>[2x]MAGRTRIPFNGVGTSVLPAYQTLSAGQYLLSPNQRFKLLLQGDGNLVIQDNGATVWVANEQQPFSSTIPLRNKKAPLAFYVQ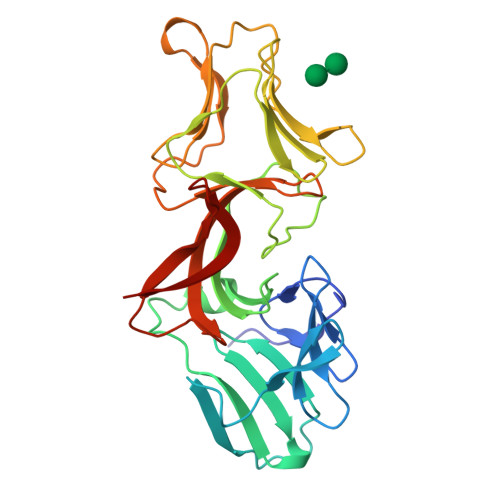YGAFLDDYSRRRVWLTDNSTFTSNDQWNRTHLVLQDDGNIVLVDSLALWNGTPAIPLVPGAIDSLLLAPGSELVQGVVYGAGASKLVFQGDGNLVAYGPNGAATWNAGTQGKGAVRAVFQGDGNLVVYGAGNAVLWHSHTGGHASAVLRLQANGSIAILDEKPVWARFGFQPTYRHIRKINPDQKPIDIWTWHF> D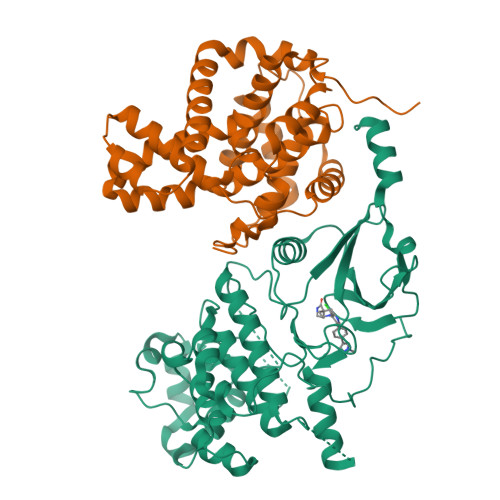KMDYDFKVKLSSERERVEDLFEYEGCKVGRGTYGHVYKAKRKDGKDDKDYALKQIEGTGISMSACREIALLRELKHPNVISLQKVFLSHADRKVWLLFDYAEHDLWHIIKFHRASKANKKPVQLPRGMVKSLLYQILDGIHYLHANWVLHRDLKPANILVMGEGPERGRVKIADMGFARLFNSPLKPLADLDPVVVTFWYRAPELLLGARHYTKAIDIWAIGCIFAELLTSEPIFHCRQEDIKTSNPYHHDQLDRIFNVMGFPADKDWEDIKKMPEHSTLMKDFRRNTYTNCSLIKYMEKHKVKPDSKAFHLLQKLLTMDPIKRITSEQAMQDPYFLEDPLPTSDVFAGCQIPYPKREFLTEEEPDDKGDKKNQQQQQGNNHTNGTGHPGNQDSSHTQGPPLKK;> KAMAGNFWQSSHYLQWILDKQDLLKERQKDLKFLSEEEYWKLQIFFTNVIQALGEHLKLRQQVIATATVYFKRFYARYSLKSIDPVLMAPTCVFLASKVEEFGVVSNTRLIAAATSVLKTRFSYAFPKEFPYRMNHILECEFYLLELMDCCLIVYHPYRPLLQYVQDMGQEDMLLPLAWRIVNDTYRTDLCLLYPPFMIALACLHVACVVQQKDARQWFAELSVDMEKILEIIRVILKLYEQWKNFDERKEMATILSKMPKPKPPPNSEGEQGPNGSQNSSYSQS2,3,5,6-tetrafluoro-N-hydroxybenzamide 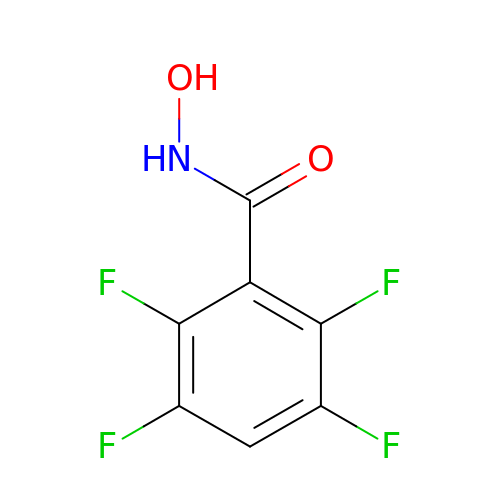| C7 H3 F4 N O2 | SOMUBBZQEJMTQV-UHFFFAOYSA-N>[6x]MGSSHHHHHHSSGLVPRGSGTENLTPQHMASMALTGTDRVKRGMAEMQKGGVIMDVVN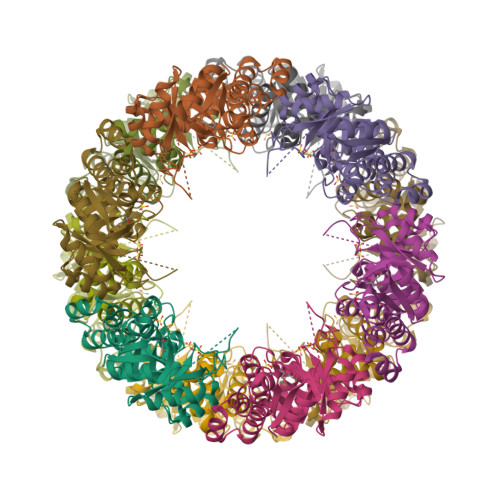AEQAKIAEAAGAVAVMALERVPADIRAAGGVARMADPTVIEEVMNAVSIPVMAKVRIGHYVEARVLEALGVDYIDESEVLTPADEEFHIDKRQFTVPFVCGCRDLGEAARRIAEGASMLRTKGEPGTGNIVEAVRHMRKVNAQIRKVVNMSEDELVAEAKQLGAPVEVLREIKRLGRLPVVNFAAGGVTTPADAALMMHLGADGVFVGSGIFKSENPEKYARAIVEATTHYEDYELIAHLSKGLGGAMRGIDIATLLPEHRMQERGW>MERDGCAGGGSRGGEGGRAPREGPAGNGRDRGRSHAAEAPGDPQAAASLLAPMDVGEEPLEKAARARTAKDPNTYKVLSLVLSVCVLTTILGCIFGLKPSCAKEVKSCKGRCFERTFGNCRCDAACVELGNCCLDYQETCIEPEHIWTCNKFRCGEKRLTRSLCACSDDCKDKGDCCINYSSVCQGEKSWVEEPCESINEPQCPAGFETPPTLLFSLDGFRAEYLHTWGGLLPVISKLKKCGTYTKNMRPVYPTKTFPNHYSIVTGLYPESHGIIDNKMYDPKMNASFSLKSKEKFNPEWYKGEPIWVTAKYQGLKSGTFFWPGSDVEINGIFPDIYKMYNGSVPFEERILAVLQWLQLPKDERPHFYTLYLEEPDSSGHSYGPVSSEVIKALQRVDGMVGMLMDGLKELNLHRCLNLILISDHGMEQGSCKKYIYLNKYLGDVKNIKVIYGPAARLRPSDVPDKYYSFNYEGIARNLSCREPNQHFKPYLKHFLPKRLHFAKSDRIEPLTFYLDPQWQLALNPSERKYCGSGFHGSDNVFSNMQALFVGYGPGFKHGIEADTFENIEVYNLMCDLLNLTPAPNNGTHGSLNHLLKNPVYTPKHPKEVHPLVQCPFTRNPRDNLGCSCNPSILPIEDFQTQFNLTVAEEKIIKHETLPYGRPRVLQKENTICLLSQHQFMSGYSQDILMPLWTSYTVDRNDSFSTEDFSNCLYQDFRIPLSPVHKCSFYKNNTKVSYGFLSPPQLNKNSSGIYSEALLTTNIVPMYQSFQVIWRYFHDTLLRKYAEERNGVNVVSGPVFDFDYDGRCDSLENLRQKRRVIRNQEILIPTHFFIVLTSCKDTSQTPLHCENLDTLAFILPHRTDNSESCVHGKHDSSWVEELLMLHRARITDVEHITGLSFYQQRKEPVSDILKLKTHLPTFSQED[2x]

Ectonucleotide pyrophosphatase/phosphodiesterase 1 (ENPP1) is an emerging therapeutic target in human cancers owing to its role in degrading cyclic GMP-AMP (cGAMP), an agonist of the stimulator of interferon genes (STING). Ectonucleotide pyrophosphatase/phosphodiesterase 1 (ENPP1), also known as PC-1, is found as a secreted protein in the extracellular matrix and as a membrane-bound protein intracellularly and on the cell surface. ENPP1 has a role in purin­ergic signalling through the hydrolysis of nucleotide triphosphates (NTPs) and cyclic nucleotides (cNMPs) to their corresponding nucleotide monophosphates (NMPs). Apart from viral poxins, ENPP1 is the only known hydrolase of cyclic GMP-AMP (cGAMP), which is a second messenger generated by cyclic GMP-AMP synthase (cGAS) as an innate immune-system response to double-stranded DNA in the cytosol.

We have determined the apo structure as well as several structures co-crystallized with natural products, natural product analogues and small-molecule inhibitors. The apo structure has only a single Zn atom in both the A and B protomers. Additional zinc was added to the gel-filtration protocol as we found that one of the two Zn atoms in the active site was either missing or not fully occupied. Asn277 adopts two distinct conformations, whereas Leu290 has a single conformer that moves slightly to accommodate bound compounds.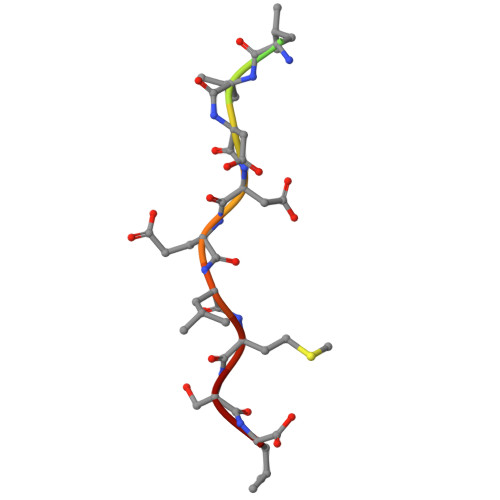> SASVSLLDDELMSL> MEESMEELEALRRKKFTTYWELKEAGSVDHTGMRL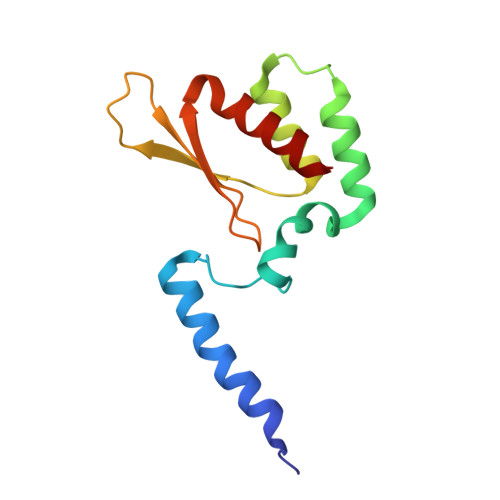CDRHNYFKNFYPTLKKEAIEAINSDEYESSKDKAMDVMSSLKITPKISEVESSSLVPLLSVELNCAFDVVLMAKETDIYDHIIDYFRTMLI>MSNKYRVRKNVLHLTDTEKRDFVRTVLILKEKGIYDRYIAWHGAAGKFHTPPGSDRNAAH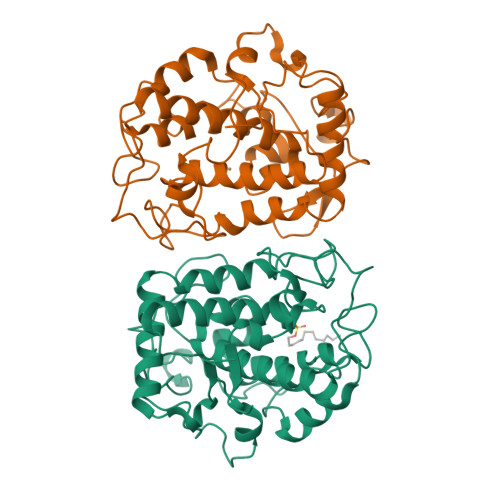MSSAFLPWHREYLLRFERDLQSINPEVTLPYWEWETDAQMQDPSQSQIWSADFMGGNGNPIKDFIVDTGPFAAGRWTTIDEQGNPSGGLKRNFGATKEAPTLPTRDDVLNALKITQYDTPPWDMTSQNSFRNQLEGFINGPQLHNRVHRWVGGQMGVVPTAPNDPVFFLHHANVDRIWAVWQIIHRNQNYQPMKNGPFGQNFRDPMYPWNTTPEDVMNHRKLGYVYDIELRKSKRSSHHHHHH[2x]> MGSNQSSSTSTKKLKAGNFDVAYQNPDKAIKGGNLKVAYQSDSPMKAQWLSGLSNDATFATMSGPGGGQDGLFFTDSGFKFI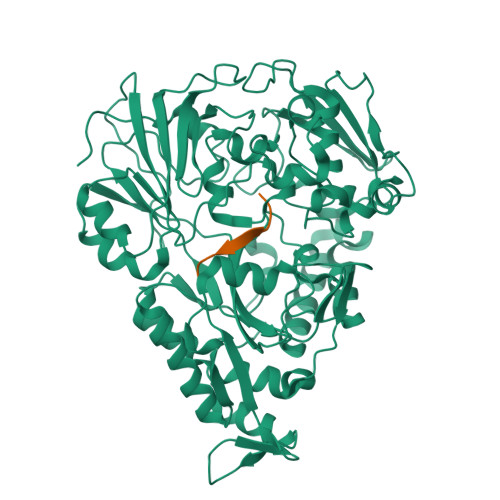KGGAADVALDKESKTATITLRKDLKWSDGSEVTAKDYEFTYETIANPAYGSDRWTDSLANIVGLSDYHTGKAKTISGITFPDGENGKVIKVQFKEMKPGMTQSGNGYFLETVAPYQYLKDVAPKDLASSPKTTTKPLVTGPFKPENVVAGESIKYVPNPYYWGEKPKLNSITYEVVSTAKSVAALSSSKYDIINGMVSSQYKQVKNLKGYKVLGQQAMYISLMYYNLGHYDAKNSINVQDRKTPLQDQNVRQAIGYARNVAEVDNKFSNGLSTPANSLIPPIFKQFTSSSVKGYEKQDLDKANKLLDEDGWKLNKSTGYREKDGKELSLVYAARVGDANAETIAQNYIQQWKKIGVKVSLYNGKLMEFNSWVDHMTTPPGANDWDITDGSWSLASEPSQQDLFSAAAPYNFGHFNDSEITKDLNDIDSAKSENPTYRKAAFVKYQEDMNKKAYVIPTNFMLNYTPVNKRVVGMTLDYGAMNTWSEIGVSSAKLATKGSIEGRHHHHHH;> SLSQLSSQS[(2~{R})-2-hexadecanoyloxy-3-[(2~{S},3~{S},4~{R},5~{R},6~{S})-6-(hydroxymethyl)-3,4,5-tris(oxidanyl)oxan-2-yl]oxy-propyl] hexadecanoate | C41 H78 O10 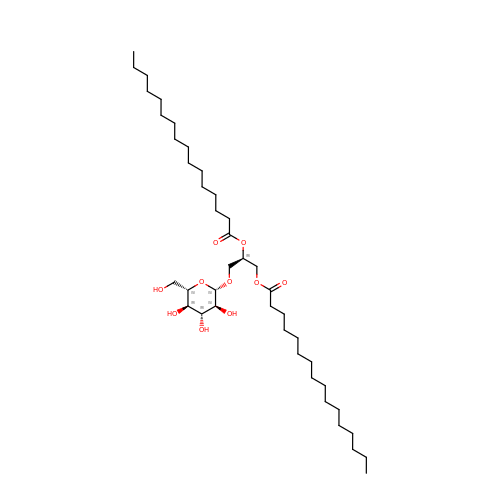| DFUALJIUMYYHRG-DWBMWBIPSA-N> PAQDNSRFVIRDRNWHPKALTPDYKTSIARSPRQALVSIPQSISETTGPNFSHLGFGAHDHDLLLNFNNGGLPIGERIIVAGRVVDQYGKP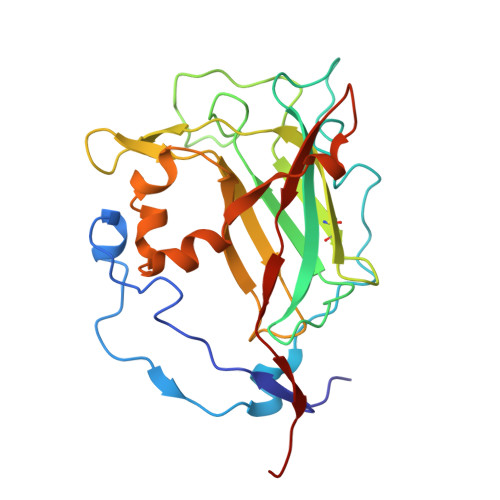VPNTLVEMWQANAGGRYRHKNDRYLAPLDPNFGGVGRCLTDSDGYYSFRTIKPGPYPWRNGPNDWRPAHIHFGISGPSIATKLITQLYFEGDPLIPMCPIVKSIANPEAVQQLIAKLDMNNANPMDCLAYRFDIVLRGQRKTHFENC> GSEGHRTLASTPALWASIPCPRSELRLDLVLPSGQSFRWREQSPAHWSGVLADQVWTLTQTEE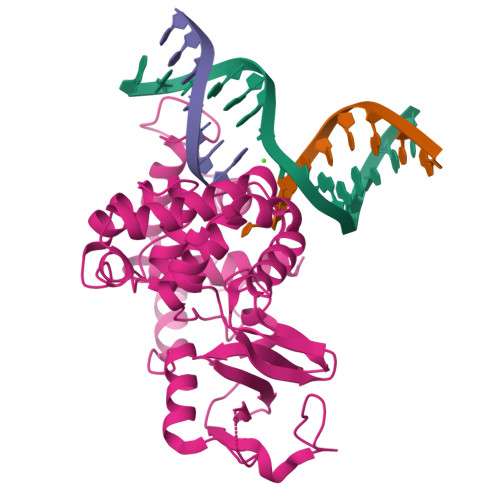QLHCTVYRGDKSQASRPTPDELEAVRKYFQLDVTLAQLYHHWGSVDSHFQEVAQKFQGVRLLRQDPIECLFSFICSSNNNIARITGMVERLCQAFGPRLIQLDDVTYHGFPSLQALAGPEVEAHLRKLGLGYRARYVSASARAILEEQGGLAWLQQLRESSYEEAHKALCILPGVGTKVADCICLMALDKPQAVPVEVHMWHIAQRDYSWHPTTSQAKGPSPQTNKELGNFFRSLWGPYAGWAQAVLFSADLRQ> TYVAPSVLESVKEKFSFEPKIRSPR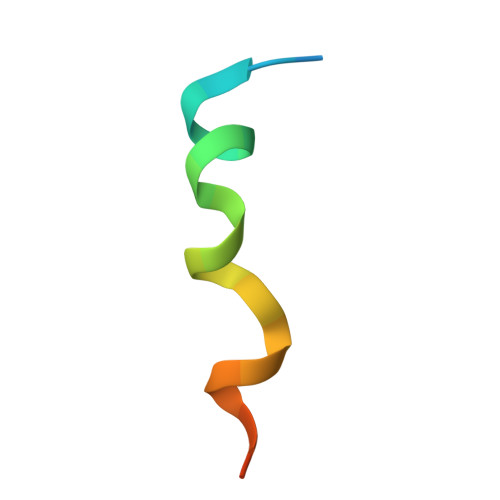R Carbonic anhydrases (CA; carbonate hydro-lyase EC 4.2.1.1) are metallo-enzymes that catalyze the reversible hydration of carbon dioxide (CO2) to bicarbonate. In this report, we describe the first crystal structure of a psychrophilic α–carbonic anhydrase from Photobacterium profundum (P. profundum), a psychrohalophile isolated from deep-sea sediment. PprCA has the characteristic carbonic anhydrase fold consisting of a ten-stranded, twisted β-sheet that is antiparallel except for 2 pairs of parallel β-strands and a few short α-helices. We also show that PprCA is functional and retains the structural core that is conserved in all carbonic anhydrases.

The final model was refined at 1.5 Angstrom resolution to Rwork of 13.9% and Rfree of 16.8%. In addition to protein atoms, the final model includes 1 zinc ion in the active site, 1 chloride ion and 342 waters. The zinc ion in active site of PprCA is coordinated by three histidine residues (His 96, His 98 and His 115) and a water molecule, denoted as Zinc-bound water. The PprCA crystal contains a monomer in the asymmetric unit. The dimer formed by the crystallographic 2-fold axis buries 751 Å2 of total surface area and superimposes well with other known bacterial CA dimers. The dimer interface of PprCA consists mainly of symmetrical polar contacts between hydrophilic side chains, water molecules and the interfacial chloride ion. A chloride ion was built into 8σ 2Fo-Fc electron density at the center of the PprCA dimer interface. The ion is completely buried in the dimer interface between electropositive surfaces created by Arg176 and Arg226 from each chain. The Cl- ion is hexa-coordinated to the amide side chains of Asn178, symAsn178 (3.43 Å) and 4 water molecules (3.1–3.26 Å), close to the ideal Cl–O distance of 3.2 Å. The chloride ion in the dimer interface of PprCA may represent halophilic adaptation by PprCA to a high salt environment.

> EWSYTGEHGTEHWGDSFATCAEGVNQTPIDINQTTQAELAPLHLDYEGQVTELVNNGHTIQANLTGKNTLTVDGKTFELKQFHFHTPSENYLKGKQYPLEAHFVHATDKGELAVVAVMFDFGPRSNNELTTLLASIPSKGQTVELKEALNPADLLPRDREYYRFNGSLTTPPCSEGVRWFVMQEPQTSSKAQTEKLQAVMGNNARPLQPLNARLILE In the present study, we conducted structural and functional analyses of the heme-responsive sensor protein PefR (porphyrin-regulated efflux regulator) from the β-hemolytic bacterium Streptococcus agalactiae, which is the most common cause of life-threatening invasive bacterial infections (e.g., septicemia, pneumonia, and meningitis) during the neonatal period. Therefore, PefR promotes the expression of these heme efflux systems in S. agalactiae in response to the intracellular heme concentration, likely by binding heme. The monomer consists of six α-helices and two β-strands containing a winged helix-turn-helix (wHTH) motif. This architecture of PefR is similar to that of the multiple antibiotic resistance regulator (MarR) family of transcriptional regulators, in which helices α2–α4 and strands β1–β2 form the DNA-binding domains.

The crystal structure of holo-PefR was determined at 1.7 Å resolution. The overall dimer structure of holo-PefR is an approximate isosceles triangle with a pseudo twofold symmetry axis. The α2, α5, and α6 helices and the α1 helix from the other subunit of the homodimer compose a hydrophobic heme pocket in the cavity. The heme is surrounded by the hydrophobic residues Pro4 and Leu 5 in the α1 helix; Leu15, Leu19, and Ala23 in the α2 helix; Leu31 and Ala32 in the loop between the α2 and α3 helices; Phe106, Leu110, and Met117 in the α5 helix; and Ile126 in the α6 helix. In the holo-PefR structure, the heme is embedded in a solvent accessible cavity and is coordinated to His114 and the N-terminal nitrogen atom on the main chain of Met1 from the other subunit of the homodimer. Heme binding in the hydrophobic pocket formed by the hydrophobic amino acid side chains changes the orientation of each subunit in the dimer, with heme coordination altering the interaction between the α1 helices from each subunit. Several polar interactions form between Arg9 and Asn13 or Glu16 in the other subunit of the dimer upon heme binding. Rigid-body motion of the α1 helix in association with heme accommodation alters the relative orientation of the DNA-binding domain in holo-PefR from the apo form, resulting in a conformational change in the DNA-binding domain (the α2, α3, and α4 helices, and the β1 and β2 strands in the wHTH region). In PefR, the hydrophobic heme pocket, together with the axial ligation of His114 and the nitrogen atom on the main chain of Met1, are responsible for its heme-binding affinity (Kd 610 nM), which is similar to the ferric heme-binding affinity of apo-myoglobin (Kd 600 nM). Apo-PefR bound 1 mol equivalent of ferric heme (protein:heme = 1:1), meaning the holo-PefR binds two hemes per dimer.

> MENPLQKARILVNQLEKYLDRYAKEYDVEHLAGPQGHLVMHLYKHPDKDMSIKDAEEILHISKSVASNLVKRMEKNGFIAIVPSKTDKRVKYLYLTHLGKQKATQFEIFLEKLHSTMLAGITKEEIRTTKKVIRTLAKNMAMEDFDSLEVLFQ>[3x]EKAVLEQ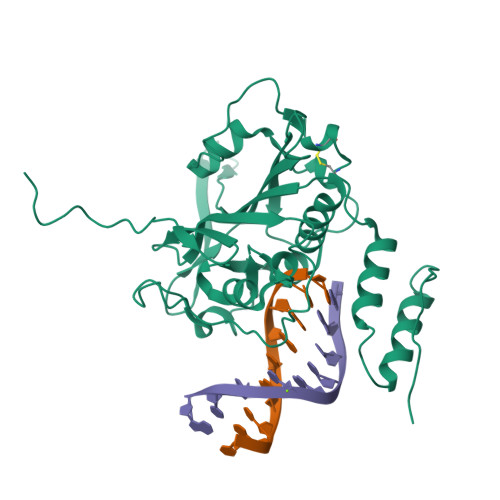FGFPLTGTEARCYTNHALSYDQAKRVPRWVLEHISKSKIMGDADRKHCKFKPDPNIPPTFSAFNEDYVGSGWSRGAMAPAGNNKFSSKAMAETFYLSNIVPQDFDNNSGYWNRIEMYCRELTERFEDVWVVSGPLTLPQTRGDGKKIVSYQVIGEDNVAVPSHLYKVILARRSSVSTEPLALGAFVVPNEAIGFQPQLTEFQVSLQDLEKLSGLVFFPHLDRTSDIRNICSVDTCKLLDFQEFTLYLSTRKIEGARSVLRLEKIMENLKNAEIEPDDYFMSRYEKKLEELKAKEQSGTQIRKPS>GPGKTDSSFIMDSDPRRCMRHHYVDSISHPLYKCSSKMVLLARCEGHCSQASRSEPLVSFSTVLKQPFRSSCHCCRPQTSKLKALRLRCSGGMRLTATYRYILSCHCE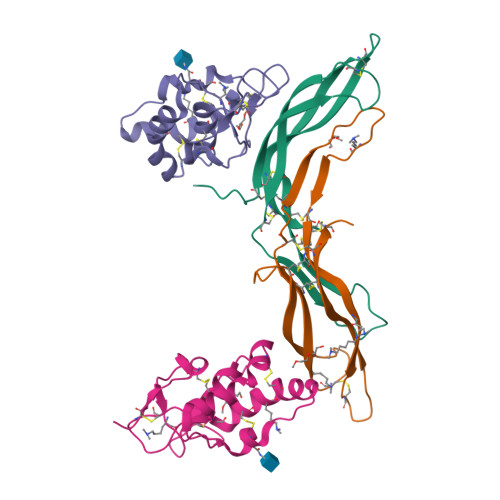ECNSGTETSQVAPA[2x];> DTGERRCDPIRISMCQNLGYNVTKMPNLVGHELQTDAELQLTTFTPLIQYGCSSQLQFFLCSVYVPMCTEKINIPIGPCGGMCLSVKRRCEPVLKEFGFAWPESLNCSKFPPQNDHNHMCMEGPGDEEVPLPHKTPIQPGEGTLEVLFQ>GPLGSESEDDKAFEENRRLRNLGSVEYIRIMSSEKSNANSRHTSKYYSGRKNFKKFQKKASQKVDGSAGSAGSENTIRILISSDPHVGYGEKDPVRGNDSFVSFNEILEIARERDVDMILLGGDIFHDNKPSRKALYQALRSLRLNCLGDKPCELELLSDTSLTTGDTAVCNINYLDPNINVAIPVFSIHGNHDDPSGDGRYSALDILQVTGLVNYFGRVPENDNIVVSPILLQKGFTKLALYGISNVRDERLYHSFRENKVKFLRPDL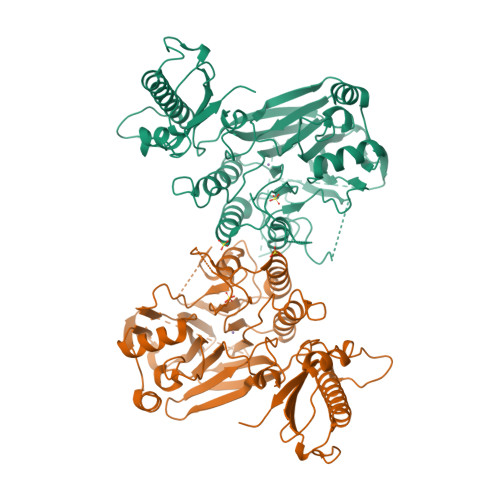YRDEWFNLLTVHQNHSAHTPTSYLPESFIQDFYDFVLWGHEHECLIDGSYNPTQKFTVVQPGSTIATSLSPGETAPKHCGILNITGKDFHLEKIRLRTVRPFIMKDIILSEVSSIPPMVENKKEVLTYLISKVEEAITEANAQWYEAQGTVPVVENEKPPLPLIRLRVDYTGGYQTENPQRFSNRFVGRVANATDVVQFYLKK[2x]>GSCKDKNEKKNYEHVNANEKNGYLASEKNELTKNKVEEHTYDYDYVVIGGGPGGMASAKEAAAHGARVLLFDYVKPSSQGTK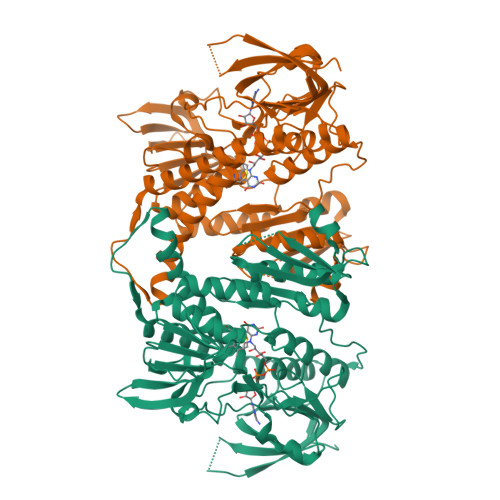WGIGGTCVNVGCVPKKLMHYAGHMGSIFKLDSKAYGWKFDNLKHDWKKLVTTVQSHIRSLNFSYMTGLRSSKVKYINGLAKLKDKNTVSYYLKGDLSKEETVTGKYILIATGCRPHIPDDVEGAKELSITSDDIFSLKKDPGKTLVVGASYVALECSGFLNSLGYDVTVAVRSIVLRGFDQQCAVKVKLYMEEQGVMFKNGILPKKLTKMDDKILVEFSDKTSELYDTVLYAIGRKGDIDGLNLESLNMNVNKSNNKIIADHLSCTNIPSIFAVGDVAENVPELAPVAIKAGEILARRLFKDSDEIMDYSYIPTSIYTPIEYGACGYSEEKAYELYGKSNVEVFLQEFNNLEISAVHRQKHIRAQKDEYDLDVSSTCLAKLVCLKNEDNRVIGFHYVGPNAGEVTQGMALALRLKVKKKDFDNCIGIHPTDAESFMNLFVTISSGLSYAAKGGCGGGKCG[2x]> ATPALRFVAVGDWGGVPNAPFHTAREMANAKEIARTVQILGADFILSLGDNFYFTGVQDINDKRFQETFEDVFSDRSLRKVPWYVLAGNHDHLGNVSAQIAYSKISKRWNFPSPFYRLHFKIPQTNVSVAIFMLDTVTLCGNSDDFLSQQPERPRDVKLARTQLSWLKKQLAA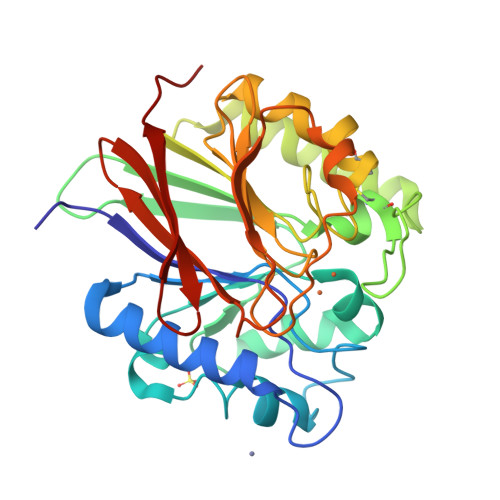AREDYVLVAGHYPVWSIAEHGPTHCLVKQLRPLLATYGVTAYLCGHDHNLQYLQDENGVGYVLSGAGNFMDPSKRHQRKVPNGYLRFHYGTEDSLGGFAYVEISSKEMTVTYIEASGKSLFKTRLPRRARP>[2x]MPSALAIFTCRPNSHPFQERHVYLDEPIKIGRSVARCRPAQNNATFDCKVLSRNHALVWFDHKTGKFYLQDTKSSNGTFINSQ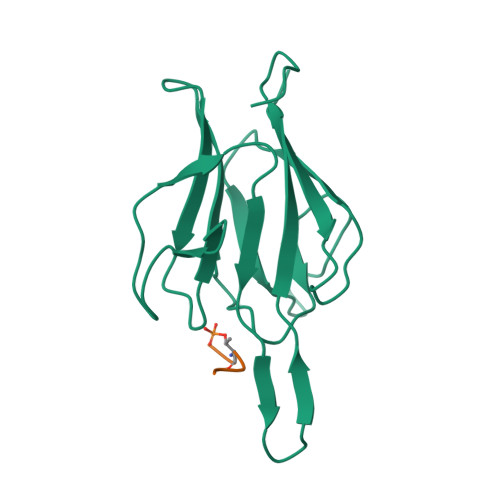RLSRGSEESPPCEILSGDIIQFGVDVTENTRKVTHGCIVSTIKLFLPDGMEARLRSD;>EEEDGTMKRN[2x]~{N}-[(1~{R})-1-(3-methoxyphenyl)ethyl]-4-pyridin-4-yl-piperidine-1-carboxamide | C20 H25 N3 O2 | 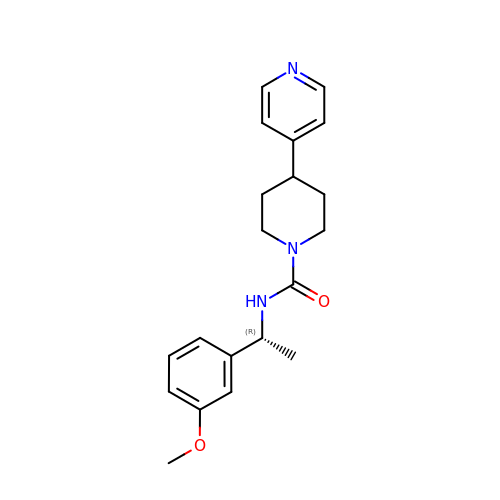TUPUYLLHTGZRRB-OAHLLOKOSA-N(2R)-3-SULFOLACTIC ACID | C3 H6 O6 S | 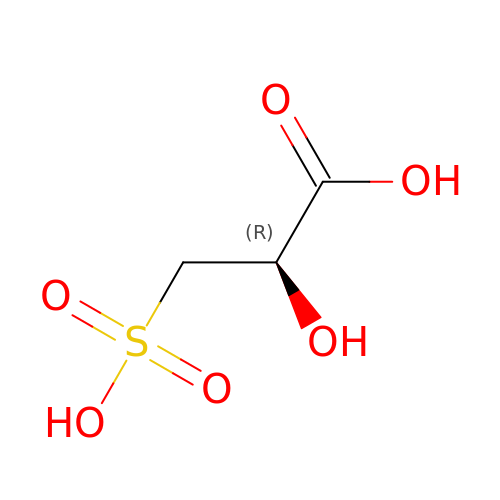CQQGIWJSICOUON-REOHCLBHSA-N>[4x]GPGSMPDIDWKQLRDKATQVAAGAYAPYSRFPVGAAALVDDGRVVTGCNVENVSYGLALCAECGVVCALHATGGGRLVALACVDGRGAPLM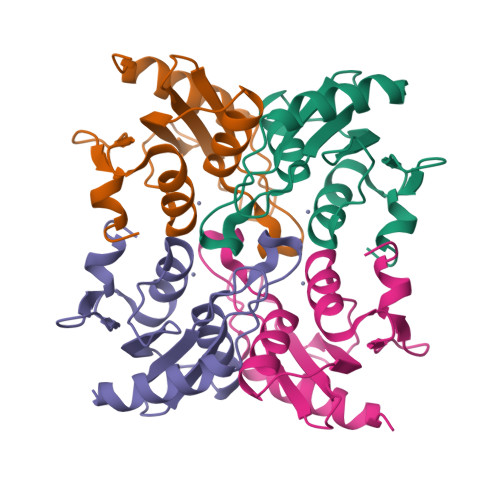PCGRCRQLLFEHGGPELLVDHLAGPRRLGDLLPEPFHADLTGEP> GSSHHHHHHSLEVLFQGPGSLIYTYKLEKYVRTKIFPKILLIPDKNRYIIKGSFRRRVPFVTDIDVVNNVYPEISRENIYDEIIKLVNNIQSDPNIILAYLSCGTDERFKISTGSSKELSNIQSLLPDNEKNEFQLVLNKYYNDQQKKLFFLNELIWDHYKLRWKPE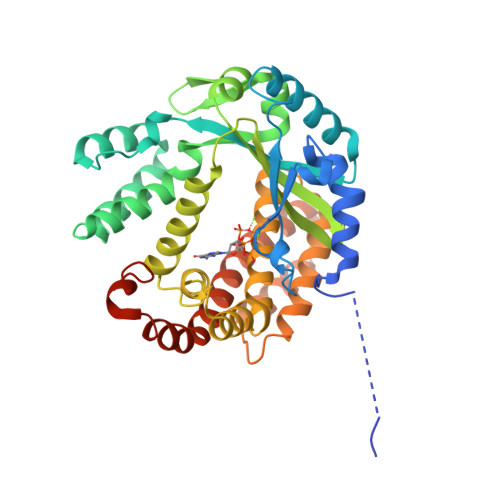DVLIGSMNLANNVSVNFRETVENNSTILLQYYVKLGSYPVGIDVVINYQKIDLTPAYKNAALYQLQLANYSREYYYMLFPLRYYFKNNQDISQRLENIIEKKYGLYKQLMVRIDDYHTLYKSGNLKIDMATNIVIGILRDIEKLPGFESDTIYQIKKVATNNSPSIKIEEWDILLKVLYQEINTAVNNKSRKYFYRYIAMVPPQDRSKNYISENQDMRLKMVN>[2x]MNILAIDIGGTMIKYGLVSFDGKILSTDKIKTEASKGLNNILNKIDNIFKRYKENNPVGIAVSGTGQINGMIGKVIGGNPIIPNWIGTNLVKILEEKYNLPIVLENDVNCVALGEKWVGAGKDLSNFICLTIGTGIGGGILLNNQLFRGENFVAGEFGHILIKKGEFEQFASTTALIRLVKERTGKTLNGKEIFDLEKKEILEYQEIISEWIENLTDGLSSIIYCFNPANIILGGGVIEQGEPLINRIKNSLFKKIGPQFKEKLNITQAKLGNNAGMIGASYLLLEKINKR

N-acetylmannosamine kinase (FnNanK) belongs to the repressor, open reading frame, kinase (ROK) superfamily of proteins. The salient unifying features of the ROK scaffold are a nucleotide-binding region in the N-terminal region, a strictly conserved catalytic aspartate residue that serves as a Schiff base during phosphoryl transfer and a zinc-binding motif that is implicated in the stability of the active site of the enzyme. Once host sialic acid has been transported across the cytoplasmic membrane (by a two-component sialic acid tripartite ATP-independent periplasmic transport system in F. nucleatum), degradation of Neu5Ac to fructose 6-phosphate starts with the conversion of sialic acid by an N-acetylneuraminate lyase (NanA), yielding N-acetyl­mannosamine (ManNAc) and pyruvate. A phosphoryl group from ATP is then transferred to ManNAc by a kinase (NanK), producing N-acetyl­mannosamine 6-phosphate (ManNAc-6-P), which in turn is converted to N-acetyl­glucosamine 6-phosphate (GlcNAc-6-P) by N-acetyl­mannosamine-6-phosphate 2-epi­merase.

In this paper, we present the crystal structure of apo FnNanK. The structure of FnNanK has one homodimer in the asymmetric unit, corresponding to a solvent content of 38%. The monomer structure has an elongated shape and is composed of two α/β domains that are connected by two hinge loops (residues 119–125 and 269–271). The putative active site is located in a large cleft between the N-terminal domain, which is made of two fragments (residues 1–118 and 272–291), and the slightly smaller C-terminal dimerization domain (residues 126–268). Forty residues of the helix cluster and connecting loops of the C-terminal domain create a 1479 Å2 dimer interface stabilized by direct hydrogen bonds and solvent-mediated hydrogen bonds. The conserved residues in hMNK (Asn516, Asp517, Arg477, Glu566, His569 and Glu588) that are required for the coordination of ManNAc are superimposable with Asn106, Asp107, Gln67, Glu156, His159 and Glu168 in FnNanK. Although FnNanK retains most of the consensus motifs unique to the ROK family, the lack of a zinc-binding site with sequence xCGxxGCx(E/D) is evident both in the sequence and structure alignments. However, FnNanK retains the highly conserved His159. We find that despite the absence of a zinc-binding motif in FnNanK, the major structural features that are implicated in enzymatic function are not compromised.(R)-4-(3-amino-4-(2,4,5-trifluorophenyl)butanoyl)piperazin-2-one | C14 H16 F3 N3 O2 | 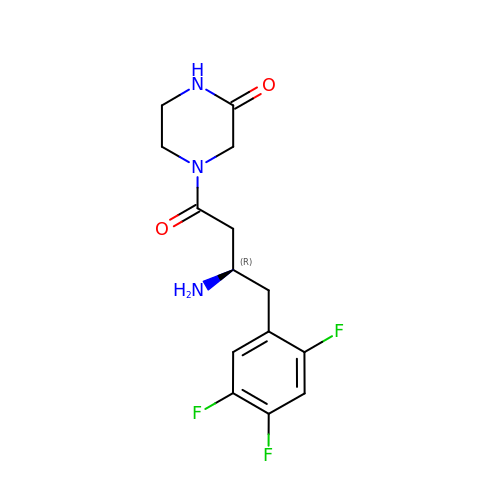SLQOQKROMQOJLJ-SECBINFHSA-N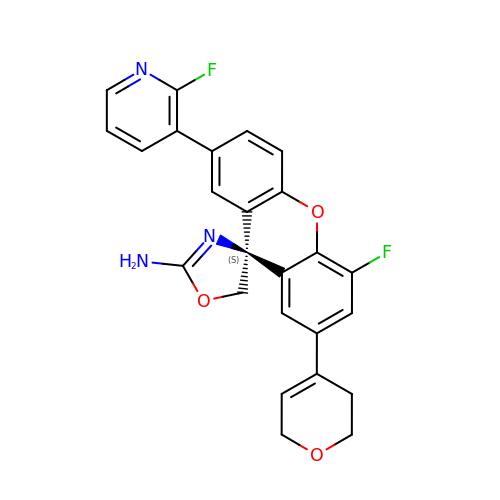(4S)-2'-(3,6-dihydro-2H-pyran-4-yl)-4'-fluoro-7'-(2-fluoropyridin-3-yl)spiro[1,3-oxazole-4,9'-xanthen]-2-amine | C25 H19 F2 N3 O3 | UBJVRJGPVXTXQB-VWLOTQADSA-N>[2x]MHRSPLAWLRLLLAAVLGAFLLGGPLHAAETAATRSPAWAQA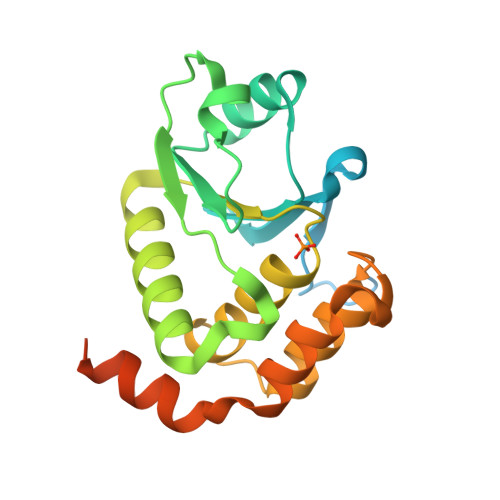VDPSINLYRMSPTLYRSALPNAQSVALLQRLQVKTVVSFIKDDDRAWLGQAPVRVLSLPTHADRVDDAEVLSVLRQLQAAEREGPVLMHCKHGNNRTGLFAAMYRIVVQGWDKQAALEEMQHGGFGDEDDMRDASAYVRGADVDGLRLAMANGECSPSRFAVCHVREWMAQALDRP> SEEQVAQDTEEVFRSYVFYRHQQEQEAEGVAAPADPEMVTLPLQPSSTMGQVGRQLAIIGDDINRRYDSEFQTMLQHLQPTAENAYEYFTKIATSLFESGINWGRVVALLGFGYRLALHV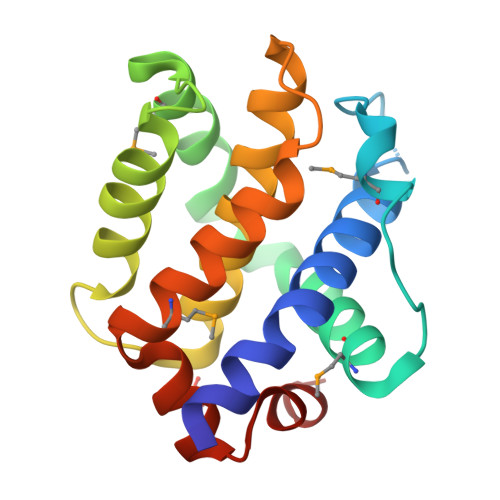YQHGLTGFLGQVTRFVVDFMLHHCIARWIAQRGGWVAALNLGN> GSAYSEKVIDHYENPRNVGSFDNNDENVGSGMVGAPACGDVMKLQIKVNDEGIIEDARFKTYGCGSAIASSSLVTEWVKGK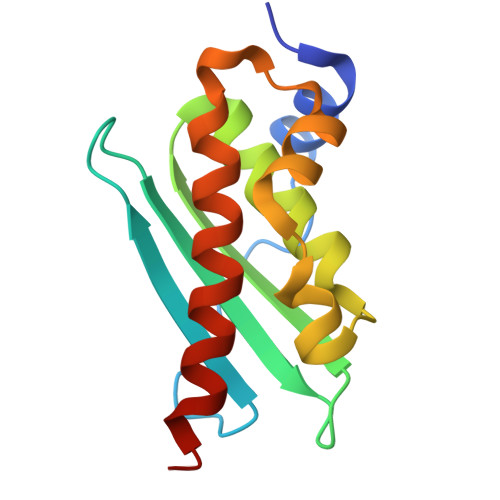SLDEAQAIKNTDIAEELELPPVKIHCSILAEDAIKAAIADYKSKREAK>MATSNVVVSRTGTGWTVDVTACNLLSDTGIKDFIVLHNAIVVSNVTYAKTTATTLTYTGAALPSNTPVEIRRKTPNSIIQLVTYGQKLSSNLWNSEIDRNIRWREEVDLNGAGLVASTPTPQNDAYGLVWAGDTFYPPTRKSVYDKIETLATKSGAVLTGATANVSPSTADNTLALATTAYVKANLADYATLVSPILTGDPRAVTTSVTDNDTSIATTAHVRAFANSRLAFNAFRGGQQGVPSLNYITTVCQFTSSAVRSGWGDNFSSNRWLVGQGGTYYVSVTCRFATTGGTPPTYMDVLLFVGLSPTGVENFVIRQQTNYPSFGYTLTWSGVLFFNTNDNVYLTYQAQAIGGGGYAVVIEDARFNAIQLS[18x];>[12x]MIRIKDFNHVITGREQPLDINEAIASYITSRYVYFKDARRVAEETWLEAWSLYSGTPEAVDHQRTQTINTVGEVNNDWRHRLNTGKAYECIETVHGYLMGALFPNREWFDLTPNNPGYANEARIIRKYLTKKFNEGKFRVSFEKYLRQLLVCGYSVMALPWRYESRPYKYNVTIKREENEYYDNSTQKANYRTVTENRVTRNAPEFECLDVFDVYLSPTSNDPNESDFIRRIKKTRADIITAIKRGYYTDIDPYDIVNMSAYEVNDRVDKLTSFQGIETNHPYCMDDIIEVVEYWGDLHLDGVSLYDVKATVIGQTLVCCEPNPFWAGKPFVVGSITELPETPYSVGLLQPNMGLLHQLNIITNQRCDNLELAIDEMWTLVQNSSLNPDEVQVAPGKVFLVDSHDDLRPIQRGGNNFVVSYQEAGLLESTIDRNTGTGNLISANASRSGERVTAAEIQAVRDAGGNRLSNIHRHIEDTSLMEILRRVYRSAQQFVTEPEMIRVSGAKPGEYLFLEVDPESLNKEYSLEPIGADFVTDATKYVRQRMDFIAFASQIPQMAERLNYEALLNDVVNHSGFDDPYSYIVKPQQPAPQPDMGATPEPQTGQAPPDEQTNPFYDIGGVSLQNAIGANIQADGANELINFTTGVNTNADQ;>[6x]MTDQFERNNIRNNEVAAEQSIQSNNFGGLNTLASPLNVPYQDSPLLLNTTVDTSGQVYKRKGTRITYTTTGTSTGCYITGFTSGLAYQFQVAKRGRDILLFQTTNDVTSLLLTKSNVWDTRAEAVRPSVVTTSEVTPRVIFATGVNKPVQLLFVEQQTTQTANGTSVVFSSADRFVNASTANCLVYVNRVLVSAPSFSYNAGTKQLTVSNLGSTVIGDVIDLVSVTWQWWAESQFWYGDRFFGSTTRFNSVSFDRVVKIPTSITTQNNGSDPYYRMRLYKQSNRTGSPNLNEVVQPQLADDWAFSDGSIYNYSVNDYPNPSPFWVVFGALVGGGQPSTVYFSRRRGLGFANGTSVQASKIDVVVNGVQRTPIYTPGSAPDSVYRNYYTYFADTTG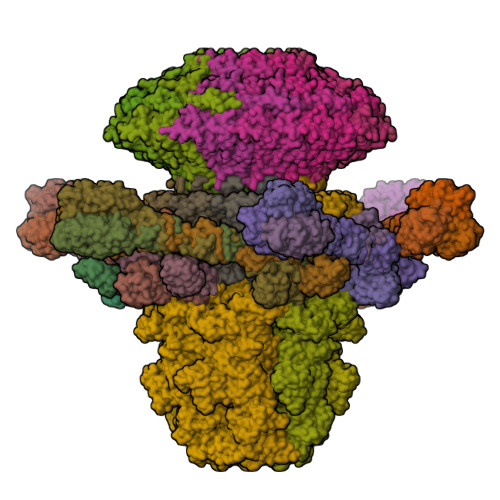AATGTSSTSLVNGIFFDAIPLGLATNDTVEASNNTNIHIGSASIATRYNYNDGSYIPAFGLGDFADYLNGYYPSVVTFFQGRLVFGGFPHRPLQVVFSNVNDNITPGRYYNSFSITDDNTALSSAFDIILNSRPDDRVVALIEWQSSLFILTRQAVFRANGGSSILSSTNRVISYVSSNGCTNSRCIVRTDFNVMYLSDTGVYNINPLVENGEYTVKELSIKIRDKFGVTREPVYEELPWMAYDSVNKQVLLGYPDVGQTNTSRYVYVYNTYRESWTEYNTPCGFNIWSTTEYTDRLLGTSVCSILYTTTSSGTPSNFIIIRWNASLYIDFIQRKTHNGSSYELTTQPAVTHTTNVNQRRYGVNFTLTRQNTAFTINPVTTVNDLYVTLDGTLLTPNVDYIKEETGYIYLLSTFSTGQTLKIASSPEGNTTPNSWYTVYVNNIRQVSPTPSAGTFTLGATNGDIINWGVNYLTIYTTPQFLWNSLGNFKRTQHAYLFLDNRDGVGVYVASDVNNGQDINQLTELYRVPINFNLSVMYNNQLDGSTSYDVMGYDSMYWDEGVFDVSSPYDQYQPYQTLKIPITGIGYAFQMLIWNHSDEYFKLGGYQIIAKQKGKRHIGRY;>MPKTTTFIQLVNKCLENIGERPVISFNNSVARKAADTVRDAITDVSYSYDWSWLTTSIIANSWINERADLGDVQSVKHVSYGSSSDGYRELTFTDERTFDAAKIYPGVGQVFTFNEYGGVRINPYPETVEEQVKYKFYVVKEATLPSVEIDVINIPDRFIQLITYNACTQLSISHLDDAQASQMWNSKYIDQLSRLRARERNTTQSGANMFKFRGTR[12x]> VVSLAGRDLLCLQDYTAEEIWTILETAKMFKIWQKIGKPHRLLEGKTLAMIFQKPSTRTRVSFEVAMAHLGGHALYLNAQDLQLRRGETIADTARVLSRYVDAIMARVYDHKDVEDLAKYATVPVINGL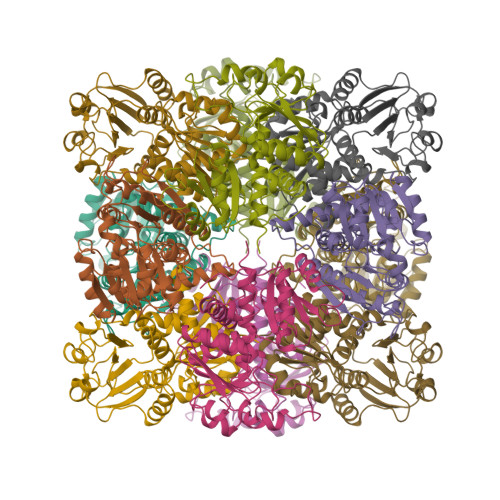SDFSHPCQALADYMTIWEKKGTIKGVKVVYVGDGNNVAHSLMIAGTKLGADVVVATPEGYEPDEKVIKWAEQNAAESGGSFELLHDPVKAVKDADVIYTDVWASMGQEAEAEERRKIFRPFQVNKDLVKHAKPDYMFMHCLPAHRGEEVTDDVIDSPNSVVWDQAENRLHAQKAVLALVMGGIKF>[3x]MLHHHHHHPMGRGTITDASGFDPLRDAEVLRKAMKGFGTDEQAIIDCLGSRSNKQRQQILLSFKTAYGKDLIKDLKSELSGNFEKTILALMKTPVLFDVYEIKEAIKGAG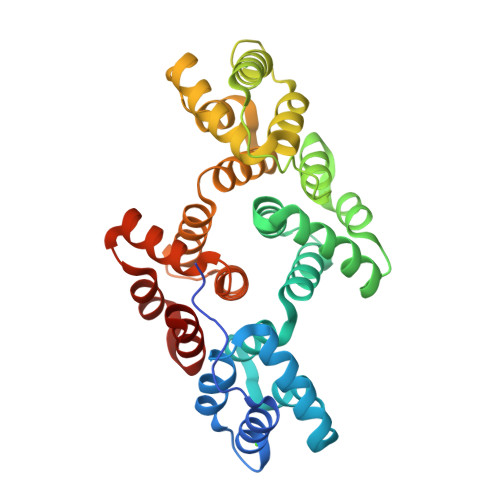TDEACLIEILASRSNEHIRELNRAYKTEFKKTLEEAIRSDTSGHFQRLLISLSQGNRDESTNVDMSLVQRDVQELYAAGENRLGTDESKFNAILCSRSRAHLVAVFNEYQRMTGRDIEKSICREMSGDLEQGMLAVVKCLKNTPAFFAERLNKAMRGAGTKDRTLIRIMVSRSELDLLDIRAEYKRMYGKSLYHDITGDTSGDYRKILLKICGGND>MVDFKLSPSQLEARRHAQAFANTVLTKASAEYSTQKDQLSRFQATRPFYREAVRHGLIKAQVPIPLGGTMESLVHESIILEELFAVEPATSITIVATALGLMPVILCDSPSLQEKFLKPFISGEGEPLASLMHSEPNGTANWLQKGGPGLQTTARKVGNEWVISGEKLWPSNSGGWDYKGADLACVVCRVSDDPSKPQDPNVDPATQIAVLLVTRETIANNKKDAYQILGEPELAGHITTSGPHTRFTEFHVPHENLLCTPGLKAQGLVETAFAMSAALVGAMAIGTARAAFEEALVFAKSDTRGGSKHIIEHQSVADKLIDCKIRLETSRLLVWKAVTTLEDEALEWKVKLEMAMQTKIYTTDVAVECVIDAMKAVGMKSYAKDMSFPRLLNEVMCYPLFEGGNIGLRRRQMQRVMALEDYEPWAATYGSS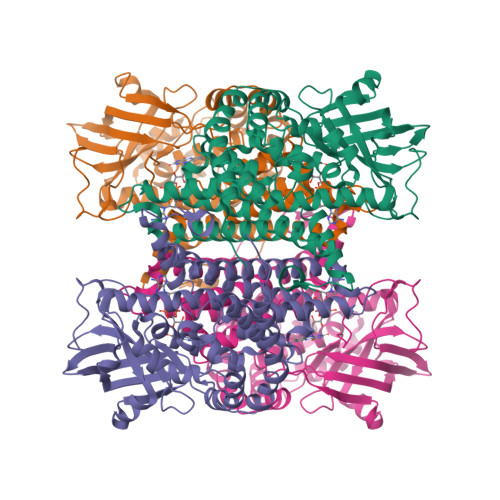KVDKSRL[4x]> MAHHHHHHSAALEVLFQKDFVLQSGQPVAIACSGSEAPVVRTSLDLLSRDLQTVLSATA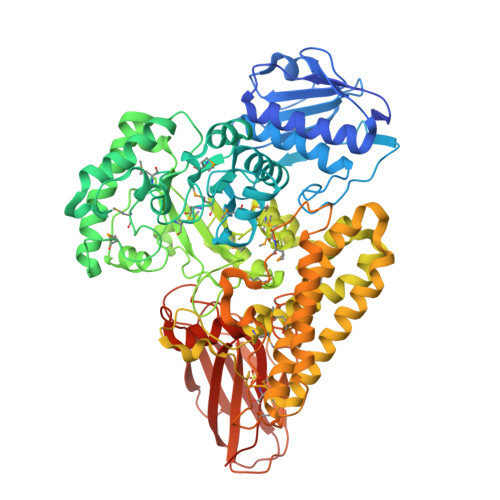HIDTNTGNIIVGTIGQSKLIEQAGIDISALKNKKQAFMLAVSEDGKLVVAGSDSHGTAYGILEISRLLGVSPWEWWADVTPEKKETFRLSGKFRELQSPSVEYRGIFINDEDWGLMPWSNKTYEPSDVKGEIGPRTNERIFELLLRLRANTYWPAMHECTLPFFLTKGNREAAKKYGIFMGASHCEPMACNAAGEWKIRGKGAYDYVNNSPAVYQFWEDRVKEVAGQEILYTLGMRGVHDGKMQGAKTVEEQKAVLDRVFVDQRGLLEKYVNKDVTQVPQVFIPYKEVLDIYHAGLQVPEDVTLMWCDDNYGYIRHFPTAEERARKGGNGVYYHVSYWGRPHDHLWLSTMSPSLIYQQMKQAYDQGIQKMWILNVGDIKPAEYQIELFMDMAWNLDKVSSEGVTAHLKHWLERELGTSCAKTILSVMQEHYRLAHIRKPEFMGNTREEEKNPVYRVVKDLPWSEREINERLNAYSELSETVEKAASKVPAGRQSAYFELVKYPVQAATQMNRKLLYAQLARHDKEDWEKSDAAYDSIAALTQHYNSLENGKWNRMMDFKPRKLPVFNRVERKAATAPMTADRKAVCQWNAAEAKKGNAIVCEGLGYESKAAEIKKGDALTFSFGNLKTDSVEVDIRLLPNHPVHGDKLRFTVSLDGAEPEVIAYETKGRSEEWKENVLRNQAIRKIVLPVTGKKSHQLVIKALDEGVILDQVMLYEVNRNSSGI>[2x]AKMAFTLADRVTEEMLADKAALVVEVVEENYHDAPIVGIAVVNEHGRFFLRPETALADPQFVAWLGDETKKKSMFDSKRAAVALKWKGIELCGVSFDLLLAAYLLDPAQGVDDVAAAAKMKQYEAVRPDEAVYGKGAKRAVPDEPVLAEHLVRKAAAIWELERPFLDELRRNEQDRLLVELEQPLSSILAEMEFAGVKVDTKRLEQMGKELAEQLGTVEQRIYELAGQEFNINSPKQLGVILFEKLQLPVLKKTKTGYSTSADVLEKLAPYHEIVENILHYRQLGKLQSTYIEGLLKVVRPATKKVHTIFNQALTQTGRLSSTEPNLQNIPIRLEEGRKIR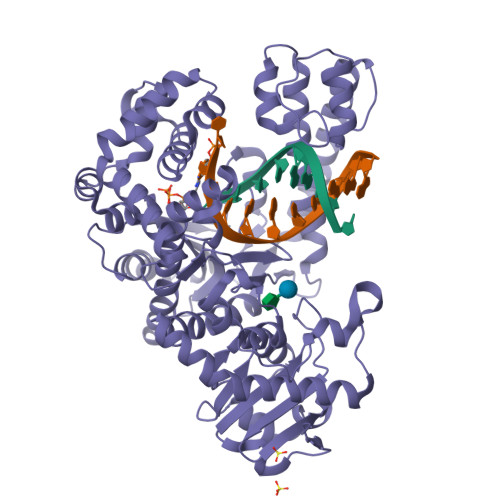QAFVPSESDWLIFAADYSQIELRVLAHIAEDDNLMEAFRRDLDIHTKTAMDIFQVSEDEVTPNMRRQAKAVNYGIVYGISDYGLAQNLNISRKEAAEFIERYFESFPGVKRYMENIVQEAKQKGYVTTLLHRRRYLPDITSRNFNVRSFAERMAMNTPIQGSAADIIKKAMIDLNARLKEERLQAHLLLQVHDELILEAPKEEMERLCRLVPEVMEQAVTLRVPLKVDYHYGSTWYDAK>[2x]MVSLVELDPAPIAEDAVVDAPYRIRNYTGFDVIISTKRQIPGASPTTEQQLPTMTLRLEDGQEAPWSFEEWEKMRESLMTESSTANSISVQLVGSGFQEVKSIRLTREGEFLFGLKPKTQQVLHKLLVEIKLGKDNIKYVTLRSPLLVENDTGIVVELGVYDAHEGHLLKIERINPGESKPAPVGAAYFKSLLVRPDPGFKYGWSSDTLWWRDLLKRPTKTLVCKSEQYGGEVFYFRLHARWDQANPLTRNYPYMRLKLTAPLTIENLLPYDFKYKIYDRVNKQEWNNFLRKGGSIPVHMVDLSHTFLLGIEMQDTPFQASEFVVINTGNADDFKKDSHLVVKDNAGMPLNLRLHYFRIPDGGGSFKVTVYSPYVILNKTGLDVSVRSKGFMQSARAAAGQTLIDVGGDGQKKARPLMFSFHNDDHRNRALLKAGDSEWSKPQSFDAIGSTTEVVLQTANRNAEIHLGVTVDSGQGKYKMVKVVTLAPRYVIHNKLGEDINIREPSSSFWIPLKHGAHRPLHWLQRGAVKQLCLCYPGVDNQWTAPFNISDLGITHLKIARAGQRQRLIRVEILMEDATIFLNLSMEQRNWPFSMRNESDTEFTFYQVNPTIEEDASEDRSGWRPVRYRLPPRSIMPYAWDFPAAKHKEICICAYNKERHVKLQEIGNLMPMKLALPNGESKTIDINVTADGPTQTLILSNYRQSKSLYRQHHHHHH

VPS13 family proteins are thought to mediate directional bulk glycerolipid transfer between organelles at contact sites, where organelles are closely apposed, effecting membrane expansion and organelle biogenesis. In yeast, Vps13p localizes to multiple contact sites in part via the so-called VPS13 adaptor binding domain (VAB), near the C-terminal end (Bean et al., 2018). The VAB, with no significant sequence similarity to any previously characterized protein domain, interacts with a Proline-X-Proline (Pro-X-Pro) motif present in receptor proteins at contact sites. Receptor proteins include the sorting nexin Ypt35p on the endosome, Spo71p on the prospore membrane, and a multipass integral membrane protein, Mcp1p, in the outer mitochondrial membrane.

Here we present the crystal structure, at 3.0-Å resolution, of the VAB from the fungus Chaetomium thermophilum, complexed to the Pro-X-Pro motif of Mcp1p from the same organism. Although we were unsuccessful in crystallizing the VAB domain by itself, we did obtain crystals of a construct comprising the VAB of C. thermophilum Vps13p (residues 1,944–2,635) N-terminally fused to the Pro-X-Pro-motif of Mcp1 (residues 15–32), PXP(Mcp1ct)-VABct. The VAB comprises six modules of the same topology arranged end to end to resemble a fishhook. There are two VAB molecules in each asymmetric unit. In the second copy, PXP-VAB1–5, we modeled only the first five repeated modules (residues 1,944–2,516), as the electron density for the sixth repeat was poor, most likely because this repeat is flexibly positioned with respect to the rest of the protein. There is strong density for the Pro-X-Pro-motif fused to the N-terminus of PXP-VAB1–5 (L17V18E19L20D21P22A23P24I25A26E27), showing that it interacts in trans with PXP-VAB1–6, binding on the acidic face of the VAB at the conserved interface between its fifth and sixth repeats. Residues L17-D21 form a short β-strand alongside and parallel to the fourth β-strand of the sixth repeat module, with the two conserved hydrophobic residues (L17 and L20) packed against hydrophobic surfaces. The two proline side chains (P22 and P24) are buried in a groove that runs along the interface. A prominent patch on the surface of the sixth module and extending to the interface between the fifth and sixth modules is highly conserved across fungi, indicating functional importance. Further, mutation of an asparagine residue at the C-terminal end of the first β-strand of the sixth repeat module of the VAB (N2521 in C. thermophilum Vps13p) abolished Pro-X-Pro binding.>MNTLRVPDILALVIFAVVFLVGVLGNALVVWVTAFEAKRTINAIWFLNLAVADFLACLALPALFTSIVQHHHWPFGGAACSILPSLILLNMYASILLLATISADRFLLVFKPAWCQRFRGAGLAWILCAVAWGLALLLTIPSALYRVVREEYFPPKVLCGVDYSHDKRRERAVAIVRLVLGFLWPLLTLTICYTFILLRTWSARETR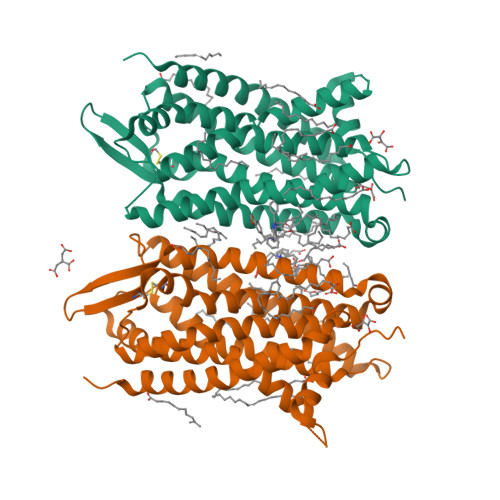STKTLKVVVAVVASFFIFWLPYQVTGIMMSFLEPSSPTFLLLKKLDSLCVSFAYINCCINPIIYVVAGQGFQGRERKSLPELLREVLTEESVVRESKAAAHHHHHHHHHH[2x]>[4x]MTTNYIFVTGGVVSSLGKGIAAASLAAILEARGLNVTIMKLDPYINVDPGTMSPIQHGEVFVTEDGAETDLDLGHYERFIRTKMSRRNNFTTGRIYSDVLRKERRGDYLGATVQVIPHITNAIKERVLEGGEGHDVVLVEIGGTVGDIESLPFLEAIRQMAVEIGREHTLFMHLTLVPYMAASGEVKTKPTQHSVKELLSIGIQPDILICRSDRAVPANERAKIALFCNVPEKAVISLKDVDSIYKIPGLLKSQGLDDYICKRFSLNCPEANLSEWEQVIFEEANPVSEVTIGMVGKYIELPDAYKSVIEALKHGGLKNRVSVNIKLIDSQDVETRGVEILKGLDAILVPGGFGYRGVEGMITTARFARENNIPYLGICLGMQVALIDYARHVANMENANSTEFVPDCKYPVVALITEWR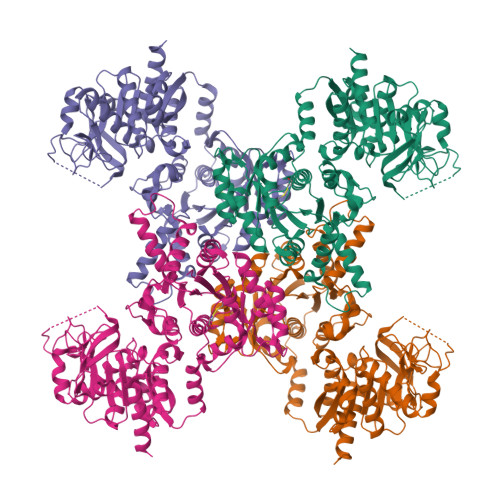DENGNVEVRSEKSDLGGTMRLGAQQCQLVDDSLVRQLYNAPTIVERHRHRYEVNNMLLKQIEDAGLRVAGRSGDDQLVEIIEVPNHPWFVACQFHPEFTSTPRDGHPLFAGFVKAASEFQKRQAK methyl 4-{[(2Z)-2-cyano-3-hydroxypent-2-enoyl]amino}-4'-fluorobiphenyl-2-carboxylate | C20 H17 F N2 O4 | 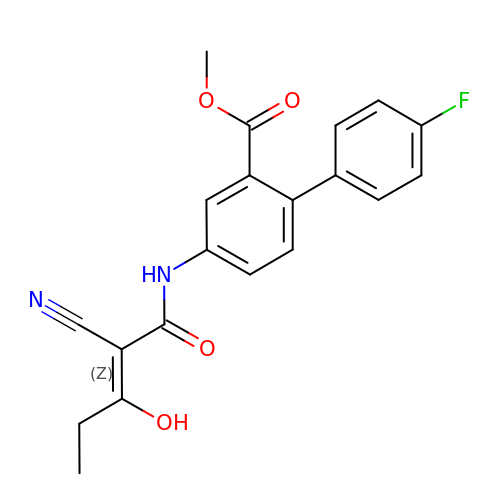IYKUBGQVTQQVJG-ZCXUNETKSA-N> MSDISFNAIPSDVRVPLTYIEFDNSNAVSGTPAPRQRVLMFGQSGSKASAAPNVPVRIRSGSQASAAFGQGSMLALMADAFLNANRVAELWCIPQGNGTGNAAVGEISLSGTAGENGSLVTYIAGQRLAVSVAAGATGAALADLLVARIKGQPDLPVTAEVRADSGDDDTHADVVLSAKFTGALSAVDVRWNYYAGETTPYGIITAFKAASGKNGNPDISASIAGMGDLQYKYIVMPYTDEPNLNLLRTELQERWGPVNQADGFAVTVLSGTYGDISTFGVSRNDHLISCMGIAGAPEPSYLYAATLCAVASQALSIDPARPLQTLTLPGRMPPAVGDRFTWSERNALLFDGISTFNVNDGGEMQIERMITMYRTNKYGDSDPSYL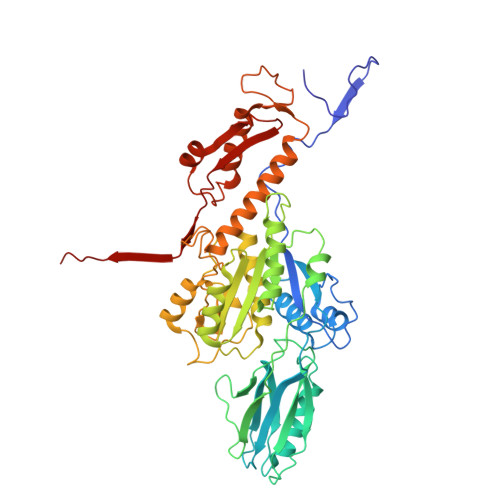NVNTIATLSYLRYSLRTRITQKFPNYKLASDGTRFATGQAVVTPSVIKTELLALFEEWENAGLVEDFDTFKEELYVARNKDDKDRLDVLCGPNLINQFRIFAAQVQFIL>[2x]MGSSHHHHHHENLYFQSNAETVAAIKT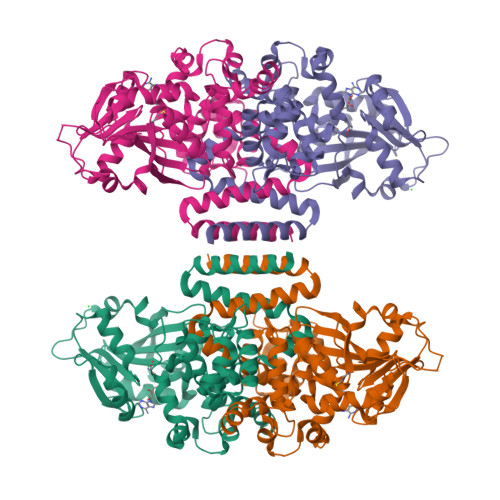LIQQLAQSTDQFGRAEINDALRELQYSLETPFDTVMRMSLDTCQVAVARIGSDLGLFKHLSQCASPQSAEELADHLGCGRELMSRLLRYMASVRMVQQTDDIKYISSNITQTLAVPGLEAGMRHAFENLWPVLMALPDFLAERKYPDIVDAKDTAFQKAFNTDQDCFHWLATQPTRIANFKVLLTDERTPNFLSTFPLEKELGSWSAEPEKALFVDIGGGMGHACIRLREKYPNQPGRVILQDLPPVLQAAQATLPLSGIESMPHNFHTPQPVQGAKFYFLRLILRDFPDHQALEILQNIVPAMDAESRIVIDDGVPPEKGARWAETGTDICIMSALGSKERTQRQWEELAAKAGLQLQALYQYTWPVVNAAMVFSLQ>[2x]GAPLPMEGVDISPKQDEGVLKVIKREGTG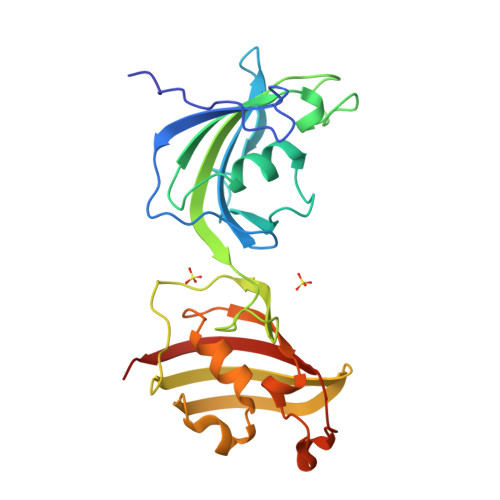TEMPMIGDRVFVHYTGWLLDGTKFDSSLDRKDKFSFDLGKGEVIKAWDIAIATMKVGEVCHITCKPEYAYGSAGSPPKIPPNATLVFEVELFEFKGEDLTEEEDGGIIRRIQTRGEGYAKPNEGAIVEVALEGYYKDKLFDQRELRFEIGEGENLDLPYGLERAIQRMEKGEHSIVYLKPSYAFGSVGKEKFQIPPNAELKYELHLKSFEKAKESWE> MEYEDLELITIWPSPTKNKLCQFIKQNLSKEHVVTQLFFIDATSSFPLSQFQKLVPPTLPENVRIYENIRINTCLDLEELSAITVKLLQILSMNKINAQRGTEDAVTEPLKIILYINGLEVMFRNSQFKSSPQRSHELLRDTLLKLRVMGNDENENASIRTLLEFPKEQLLDYYLKKNNNTRTSSVRSKRRRIKNGDSLAEYIWKYYADSLF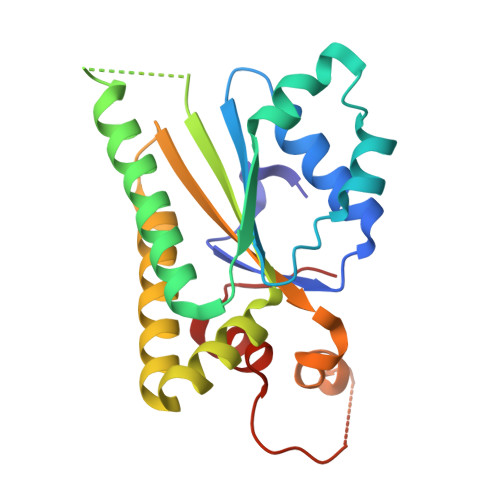E> MKHLHRFFSSDASGGIILIIAAILAMIMANSGATSGWYHDFLETPVQLRVGSLEINKNMLLWINDALMAVFFLLVGLEVKRELMQGSLASLRQAAFPVIAAIGGMIVPTLLYLAFNYADPITREGWAIPAATDIAFALGVLALLGSRVPLALKIFLMALAIIDDLGAIIIIALFYTNDLSMASLGVAAVAIAVLAVLNLCGARRTGVYILVGVV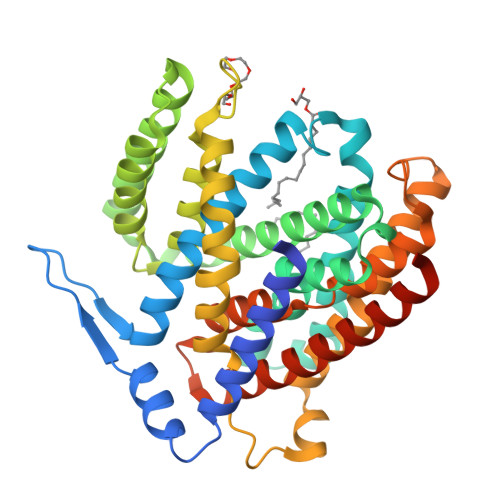LWTAVLKSGVHATLAGVIVGFFIPLKEKHGRSPAKRLEHVLHPWVAYLILPLFAFANAGVSLGGVTLDGLTSILPLGIIAGMLIGKPLGISLFCWLALRLKLAHLPEGTTYQQIMVVGILCGIGFTMSIFIASLAFGSVDPELINWAKLGILVGSISSAVIGYSWLRVRLRPSVGSENLYFQ>DWPVYHRIDGPIVMIGFGSIGRGTLPLIERHFAFDRSKLVVIDPSDEARKLAEARGVRFIQQAVTRDNYRELLVPLLTAGPGQGFCVNLSVDTSSLDIMELARENGALYIDTVVEPWLGFYFDPDLKPEARSNYALRETVLAARRNKPGGTTAVSCCGANPGMVSWFVKQALVNLAADLGVTGEEPTTREEWARLAMDLGVKGIHIAERDTQRASFPKPFDVFVNTWSVEGFVSQGLQPAELGWGTFERWMPDNARGHDSGCGAGIYLLQPGANTRVRSWTPTAMAQYGFLVTHNESISIADFLTVRDAAGQAVYRPTCHYAYHPCNDAVLSLHEMFGSGKRQSDWRILDETEIVDGIDELGVLLYGHGKNAYWYGSQLSIEETRRIAPDQNATGLQ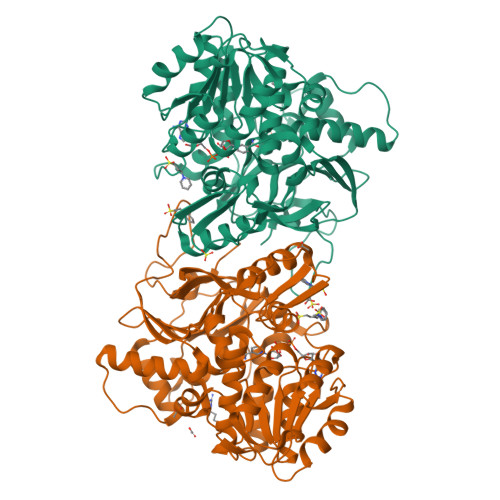VSSAVLAGMVWALENPNAGIVEADDLDFRRCLEVQTPYLGPVVGVYTDWTPLAGRPGLFPEDIDTSDPWQFRNVLVRD[2x]>MALEPLKVEKFATANRGNGLRAVTPLRPGELLFRSDPLAYTVCKGSRGVVCDRCLLGKEKLMRCSQCRVAKYCSAKCQKKAWPDHKRECKCLKSCKPRYPPDSVRLLGRVVFKLMDGAPSESEKLYSFYDLESNINKLTEDKKEGLRQLVMTFQHFMREEIQDASQLPPAFDLFEAFAKVICNSFTICNAEMQEVGVGLYPSISLLNHSCDPNCSIVFNGPHLLLRAVRDIEVGEELTICYLDMLMTSEERRKQLRDQYCFECDCFRCQTQDKDADMLTGDEQVWKEVQESLKKIEELKAHWKWEQVLAMCQAIISSNSERLPDINIYQLKVLDCAMDACINLGLLEEALFYGTRTMEPYRIFFPGSHPVRGVQVMKVGKLQLHQGMFPQAMKNLRLAFDIMRVTHGREHSLIEDLIL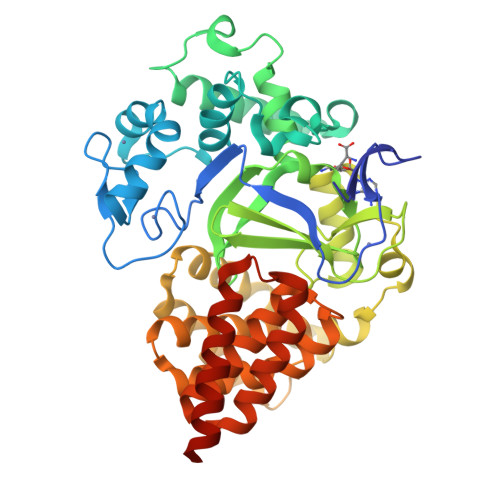LLEECDANIRASEGHHHHHH[2x]> MDQECIENYAKVNGIYIYYKLCKAPEEKAKLMTMHGGPGMSHDYLLSL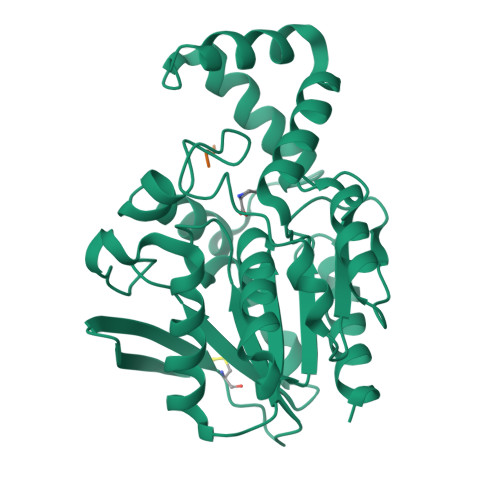RDMTKEGITVLFYDQFGCGRSEEPDQSKFTIDYGVEEAEALRSKLFGNEKVFLMGSAYGGALALAYAVKYQDHLKGLIVSGGLSSVPLTVKEMNRLIDELPAKYRDAIKKYGSSGSYENPEYQEAVNYFYHQHLLRSEDWPPEVLKSLEYAERRNVYRIMNGPNEFTITGTIKDWDITDKISAIKIPTLITVGEYDEVTPNVARVIHEKIAGSELHVFRDCSHLTMWEDREGYNKLLSDFILKHL;> PLGG>[2x]MGSSHHHHHHSSPRLFMLSSTSSDALRQTARQLATWVEEHQDCVAASDLAYTLARGRAHRPV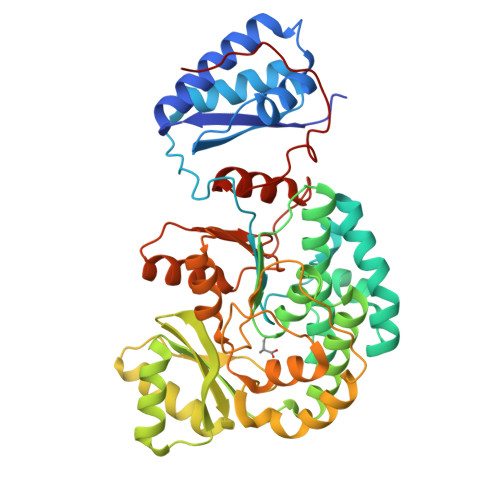RTAVVAANLPELVEGLREVADGDALYDAAVGHGDRGPVWVFSGQGSQWAAMGTQLLASEPVFAATIAKLEPVIAAESGFSVTEAITAQQTVTGIDKVQPAVFAVQVALAATMEQTYGVRPGAVVGHSMGESAAAVVAGALSLEDAARVICRRSKLMTRIAGAGAMGSVELPAKQVNSELMARGIDDVVVSVVASPQSTVIGGTSDTVRDLIARWEQRDVMAREVAVDVASHSPQVDPILDDLAAALADIAPMTPKVPYYSATLFDPREQPVCDGAYWVDNLRNTVQFAAAVQAAMEDGYRVFAELSPHPLLTHAVEQTGRSLDMSVAALAGMRREQPLPHGLRGLLTELHRAGAALDYSALYPAGRLVDAPLPAWGS> PAPQTSIELFLIVDHSMYAKYNSNSSKITTTLKARVNIMNAIYSSLNLVITLSGIEMWSAADLITVQSSSRNTLKLFASWRETDLLKRTSNDNAQLLTATNFNGNTVGLAYLKTMCNSKYSVGLIQDHSAIPLLMAV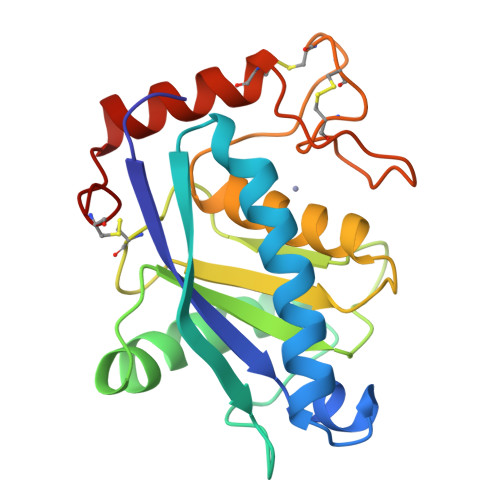TMAHELGHNLGMNHDGAGCSCATCIMAPVLSSGPAKSFSDCSKHDYQSFLTIHKPQCLLN> MMKTTISVIKADIGSLAGHHIVHPDTMAAANKVLASAKEQGIILDYYITHVGDDLQLIMTHTRGELDTKVHETAWNAFKEAAKVAKDLGLYAAGQDLLSDSFSGNVRGLGPGVAEMEIEERASEPIAIFMADKTEPGAYNLPLYKMFADPFNTPGLVIDPTMHGGFKFEVLDVYQGEAVMLSAPQEIYDLLALIGTPARYVIRRVYRNEDNLLAAVVSIERLNLIAGKYVGKDDPVMIVRLQHGLPALGEALEAFAFPHLVPGWMRGSHYGPLMPVSQRDAKATRFDGPPRLLGLGFNVKNGRLVGPTDLFDDPAFDETRRLANIVADYMRRHGPFMPHRLEPTEMEYTTLPLILEKLKDRFKKESDVYKAKESIYA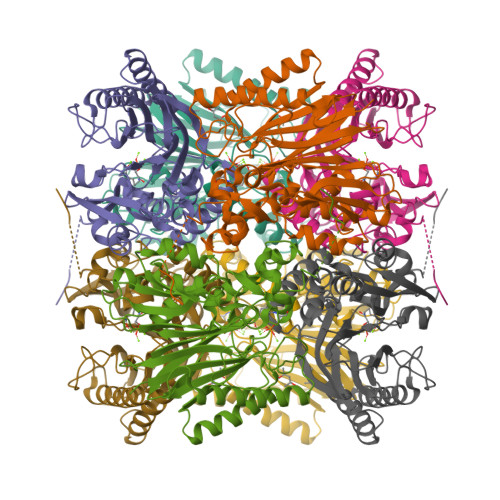KEESQGHD> QEPGSGIGYPYDNNTLPYVAPGPTDSRAPCPALNALANHGYIPHDGRAISRETLQNAFLNHMGIAN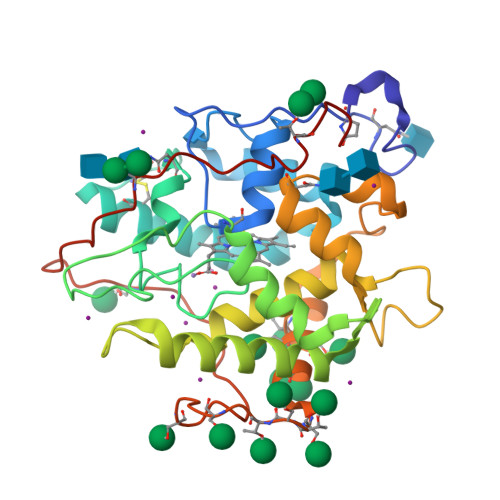SVIELALTNAFVVCEYVTGSDCGDSLVNLTLLAEPHAFEHDHSFSRKDYKQGVANSNDFIDNRNFDAETFQTSLDVVAGKTHFDYADMNEIRLQRESLSNELDFPGWFTESKPIQNVESGFIFALVSDFNLPDNDENPLVRIDWWKYWFTNESFPYHLGWHPPSPAREIEFVTSASSAVLAASVTSTPSSLPSGAIGPGAEAVPLSFASTMTPFLLATNAPYYAQDPTLGPND The virulence of P. gingivalis is dependent on secreted cysteine proteases called gingipains (RgpA, RgpB, and Kgp) that are essential for corruption of the host immune system and acquisition of nutrients and heme – a vital growth factor and source of black pigmentation of colonies on blood agar. Gingipains are synthesized with a typical N-terminal signal peptide targeting them to the Sec translocon and are exported through the OM via a novel secretion system referred to as “Por Secretion System; PorSS” or following the naming convention, Type IX Secretion System (T9SS)7. Translocation of gingipains from the periplasm across the OM is dependent on a conserved C-terminal domain (CTD), which appears to be important for secretion of the proteins and in particular, truncation of the last few C-terminal residues of this domain leads to accumulation of gingipains in the periplasm. Here, we show for the first time that the OM translocation signal, a conserved CTD of RgpB, has a typical Ig-like fold encompassing seven antiparallel β-strands organized in two β-sheets that are packed against each other in a β-sandwich.

In addition to the rIgSF-CTD tandem of the Ig-like folded domains, we solved the structure of the rCTD alone. Crystals were obtained from a fragment encompassing residues S664–K736, which crystallized in the hexagonal space group, P65. The structure was solved to 1.9 Å resolution and the Fourier map enabled us to trace residues K672–K736. The asymmetric unit contained a dimer of rCTD molecules (approximately 75 Å × 21 Å × 14 Å) in a side-to-side arrangement, with the monomers related to each other by a twofold axis. Superimposition of one monomer with the corresponding domain in the rIgSF-CTD tandem revealed that the conformations of strands s1–s6 (corresponding to the 55 N-terminal residues) of the rCTD were very similar. However, a significant difference was observed between the polypeptide chain encompassing residues V717–V735 corresponding to the s6-s7 loop and the last strand (s7) of the CTD. In this structure, strand 7 was swapped between the two monomers and constituted the primary interface between them. Thus, in this conformation, the s6-s7 loop, instead of a turn, adopts an extended conformation along the s6 main axis, bringing s7 to interact with the neighboring monomer. The equivalent region from the neighboring monomer then occupies the space generated by this movement in an identical manner. This domain swap, as a consequence, generates an antiparallel β-sheet between strands s6 and s7, as occurs in the absence of swapping, that has the same backbone and side chain set of interactions, with the only differences being the monomer that provides s7 and the conformation of the s6-s7 loop. Of note, this C-terminal export signal is the same region of the protein that strand swapping occurs in our rCTD dimer.

>[2x]IADVANDKPYTVAVSGKTITVESPAAGLTIFDMNGRRVATAKNRMVFEAQNGVYAVRIATEGKTYTEKVIVK> GSKEGEYIKLKVIGQDSSEIHFKVKMTT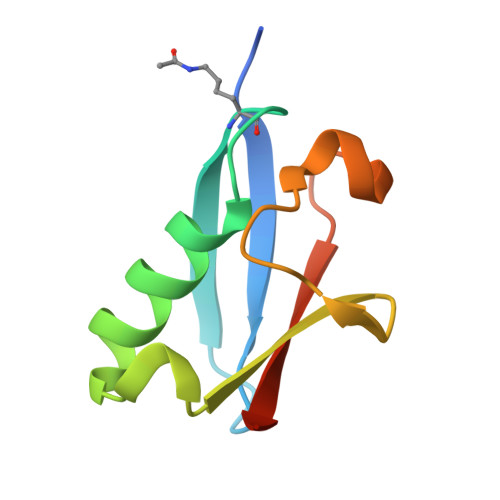HLKKLKESYAQRQGVPMNSLRFLFEGQRIADNHTPKELGMEEEDVIEVYQEQTGG> SKLLDNLRDTVRKFLTGSSSYDKAVEDFIKELQKSLISADVNVKLVFSLTNKIKERLKNEKPPTYIERREWFIKIVYDELSNLFGGDKEPKVIPDKIPYVIMLVGVQGTGKATTAGKLAYFYKKKGFKVGLVGADVYRPAALEQLQQLGQQIGVPVYGEPGEKDVVGIAKRGVEKFLSEKMEIIIVDTAGRHGYGEEAALLEEMKNIYEAIKPDEVTLVI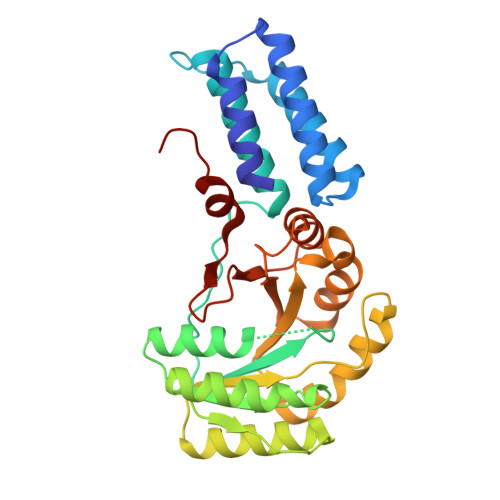DASIGQKAYDLASKFNQASKIGTIIITKMDGTAKGGGALSAVAATGATIKFIGTGEKIDELEVFNPRRFVARLHHHH> GSPEEWLDILGNGLLRKKTLVPGPPGSSRPVKGQVVTVHLQTSLENGTRVQE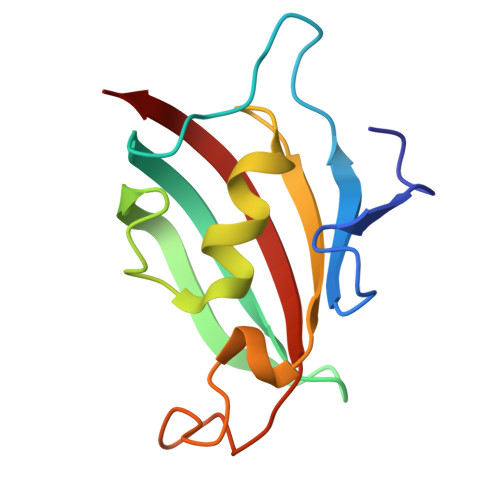EPELVFTLGDCDVIQALDLSVPLMDVGETAMVTADSKYCYGPQGRSPYIPPHAALCLEVTLKTAVD> G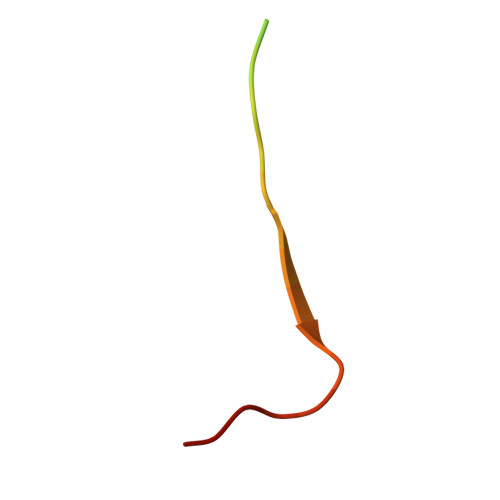PGGSGGPSPPPTWPHLQLCYLQPPPV> GSGSGSGRGGSCLAAAHHR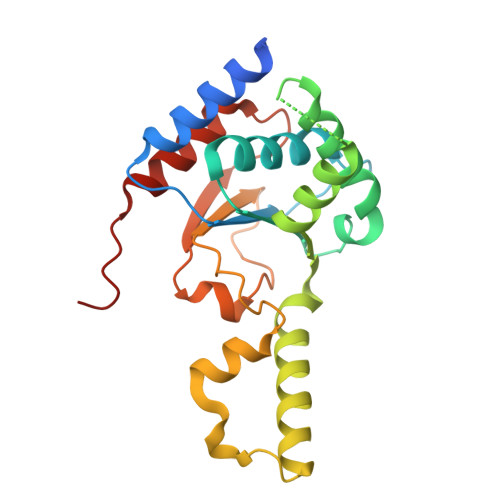MRWRADGRSLEKLPVHMGLVITEVEQEPSFSDIASLVVWCMAVGISYISVYDHQGIFKRNNSRLMDEILKQQQELLGLDCSKDKDDQVLNCHLAVKVLSPEDGKADIVRAAQDFCQLVAQKQKRPTDLDVDTLASLLSSNGCPDPDLVLKFGPVDSTLGFLPWHIRLTEIVSLPSHLNISYEDFFSALRQYAACEQRLGK>[2x]GMSEAPHLTFDLDTPGVSTGHLVVPKGADCEALSLPVFSCNRGEGPSLLITGGNHGNELQGPILARRLVKWLPEAQRCGRIIIVPEINPLAVQAWTRNTPIDGKNLNRVFPGRSDGSVSERIADAISRLLLPVVDTVLDLHSFGPTWDCAPSIISHP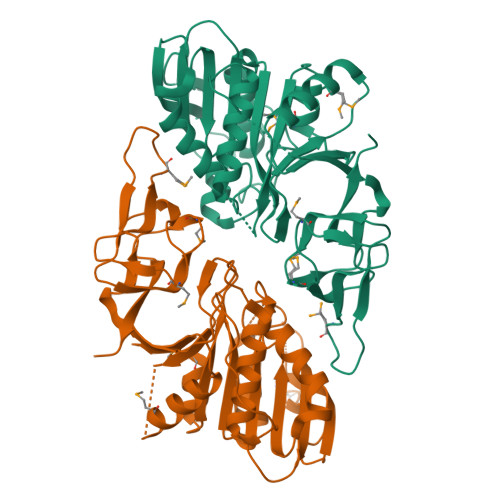IADIDQMTKTVSISKAFKLPVTLLWEHNETDGMFDTLVHRQGKTFICTEFGGGVVSAEALTIYEAGVRNGLIALGLVKGKAEYPTFRQQKTGQTLETTSSDQLKSPSPGIFEPRCSVMDEVEQGDVVGVLHPMGSLSAASIDIRAQSKSTVFAIRSAMYVQGNEEVAILARPLAR> SRKIIHVDMDCFFAAVEMRDNPALRDIPIAIGGSRERRGVISTANYPARKFGVRSAMPTGMALKLCPHLTLLPGRFDAYKEASNHIREIFSRYTSRIEPLSLDEAYLDVTDSVHCHGSATLIAQEIRQTIFNELQLTASAGVAPVKFLAKIASDMNKPNGQFVITPAEVPAFLQTLPLAKIPGVGKVSAAKLEAMGLRTCGDVQKCDLVMLLKRFGKFGRILWERSQGIDERDVNSERLRKSVGVERTMAEDIHHWSECEAIIE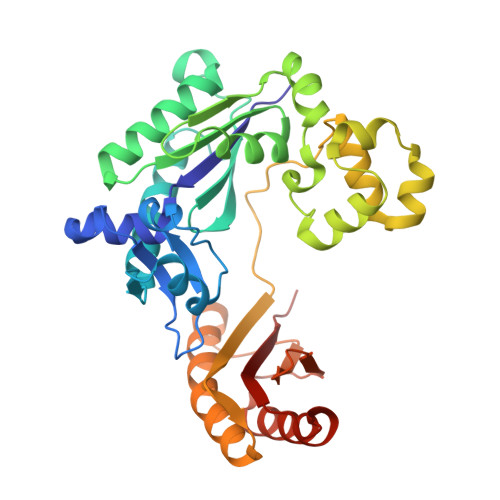RLYPELERRLAKVKPDLLIARQGVKLKFDDFQQTTQEHVWPRLNKADLIATARKTWDERRGGRGVRLVGLHVTLLD Peptidoglycan amidases are key hydrolytic enzymes that are needed to break the peptidoglycan layer during cell division to allow for separation of daughter cells. All the three division-associated amidases have overlapping enzymatic functions in hydrolyzing the peptidoglycan amide bond between the sugar and the first amino acid of the peptide cross-link. In their resting states, zinc-dependent peptidoglycan amidases such as AmiB and AmiC adopt autoinhibited conformations in which their active sites are blocked by an alpha helix containing a conserved glutamate residue which binds to the active-site zinc. The activators share a common motif, the LytM domain, which forms the proposed site of amidase binding and activation.

Crystals of AmiA diffract to a resolution of 2.4 Å and contain two molecules per asymmetric unit. Each AmiA monomer consists of a single globular domain with a six-membered beta sheet and six alpha helices. The AmiA active site is composed of a single zinc atom that is held in place by two histidine residues (His65 and His133), an aspartate (Asp135), and two glutamates (Glu80 and Glu167). Similar to AmiB and AmiC, the AmiA active-site zinc is not accessible to peptidoglycan substrates due to the presence of an alpha helix that occludes the active site; we term this feature the “blocking helix” (red). As demonstrated in subsequent sections, the blocking helix has a role in autoinhibiting the activity of AmiA and forms part of a larger regulatory domain (residues 151–194) which includes a second alpha helix that constitutes the binding site for EnvC. We define the latter feature as the “interaction helix” (blue). The interaction helix is also notable for possessing five solvent-facing hydrophobic residues (Leu184, Leu185, Val188, Leu189, Leu192) and is the only feature for which we identify meaningful conformational differences between the two AmiA molecules observed in the crystal structure. In one chain, the interaction helix is well defined, while in the other, the corresponding electron density is smeared out, consistent with thermal motion. We further assessed the dynamics of AmiA by plotting the B-factors from each monomer against sequence and performing molecular dynamics simulations. Both the experimental data and simulations consistently show that the regulatory domain is much more dynamic than the rest of the protein. The overall structure of AmiA is consistent with an autoinhibited form of the enzyme in which the active-site zinc is occluded by the blocking helix, while a potential protein interaction site remains exposed to solvent ready for activation.

>[2x]MKDELLKTSNGHSKPKAKKSGGKRVVVLDPGHGGIDTGAIGRNGSKEKHVVLAIAKNVRSILRNHGIDARLTRSGDTFIPLYDRVEIAHKHGADLFMSIHADGFTNPKAAGASVFALSNRGASSAMAKYLSERENRADEVAGKKATDKDHLLQQVLFDLVQTDTIKNSLTLGSHILKKIKPVHKLHSRNTEQAAFVVLKSPSVPSVLVETSFITNPEEERLLGTAAFRQKIATAIAEGVISYFHWFDNQKAHSKKRLEHHHHHH> ADNQENDSTNVHNTKLASTSAENAIEKEQITTFHDVETPNRIDTPMAQDTSSARSMDDTHSIIQFLQRPVLIDNIEIVAGTTADNNTALSRYVL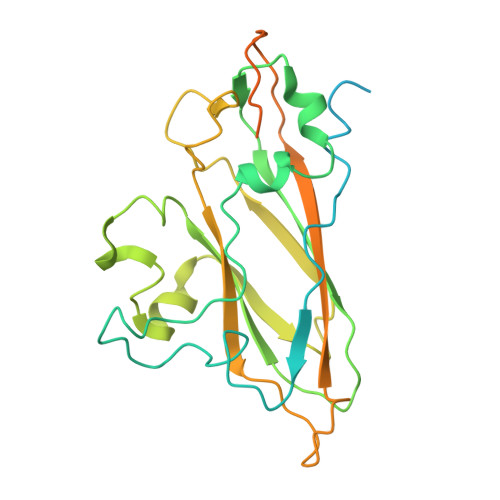DRTNPQKYIKQWTLPSTVLKAGGKAQKLANFKYLRCDVQVKIVLNANPFIAGRLYLAYSPYDDKVAPERRIIYTSRAGVTGYPGVELDFQLDNSVEMTIPYASFQEAYDLVSGNEDFVQLYLFTIAPVLGPSAESANSKVDLSVYMWLDNISLVIPTYRLNPNLPTGQTLTRIVQNSDSDKLKEALKIAKSKNPSGYKYIMGVLEQYNPSVKQVSMQ>MFTGSIVAIVTPMDEKGNVCRASLKKLIDYHVASGTSAIVSVGTTGEWATLNHDEHADVVMMTLDLADGRIPVIAGTGANATAEAISLTQRFNDSGIVGCLTVTPYYNRPSQEGLYQHFKAIAEHTDLPQILYNVPSRTGCDLLPETVGRLAKVKNIIGIKEAT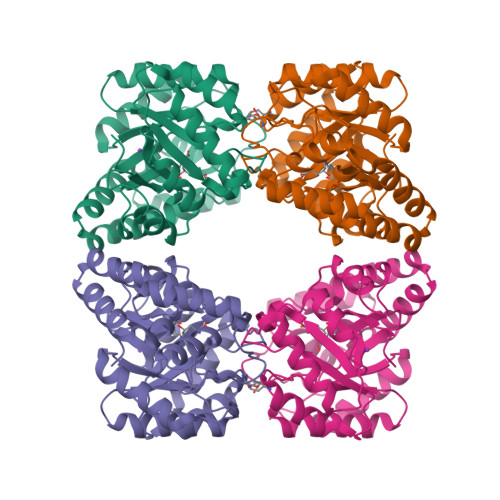GNLTRVNQIKELVSDDFVLLSGDDASALDFMQLGGHGVISVTANVAARDMAQMCKLAAEGHFAEARVINERLMPLHNKLFVEPNPIPVKWACKELGLVATDTLRLPMTPITDSGRETVRAALKHAGLL[2x]>MAHHHHHHKPQEVVRLGDIQMANHLPFVLFGGMNVLESKDLAFEIAETYIDICKRLDIPYVFKASFDKANRSSLHSFRGPGLEKGIEW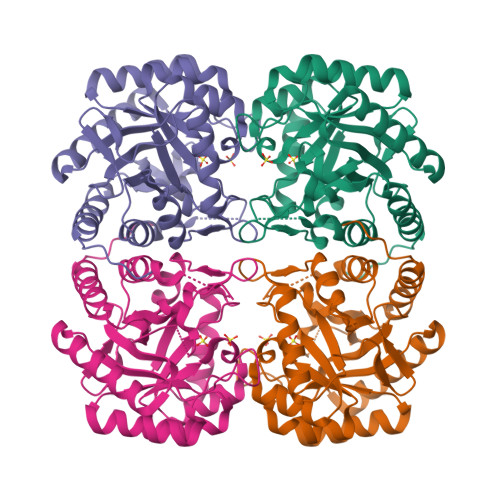LGDIKKHFNVPIITDVHEPYQAAPVAEVADIIQLPAFLSRQTDLVEAMAKTQAIINIKKAQFLAPHEMRHILHKCLEAGNDKLILCERGSAFGYNNLVVDMLGFDIMKEMNVPVFFDVTHALQTPGGRSDSAGGRRAQITTLARAGMATGLAGLFLESHPDPDKAKCDGPSALRLSQLEPFLAQLKELDTLVKGFKKLDTH[2x]>[8x]MAELACFCYPHLENDSYKFIPFNNLAIKAMLTAKVDKKDMDKFYDSIIYGIAPPPQFKKRYNTNDNSRGMNFETIMFTKVAMLICEALNSLKVTQANVSNVLSRVVSIRHLENLVIRKENPQDILFHSKDLLLKSTLIAIGQSKEIETTITAEGGEIVFQNAAFTMWKLTYLEHQLMPILDQNFIEYKVTLNEDKPISDVHVKELVAELRWQYNKFAVITHGKGHYRIVKYSSVANHADRVYATFKSNVKTGVNNDFNLLDQRIIWQNWYAFTSSMKQGNTLDVCKRLLFQKMKPEKNPFKGLSTDRKMDEVS

In RVs, the viral RNA chaperone protein NSP2 facilitates sequence-specific, intersegment RNA–RNA interactions to ensure robust assembly of complete viral genomes. NSP2 is a multivalent, nonspecific RNA chaperone with high nanomolar affinity for single-stranded (ss) RNA. The CTR of NSP2 consists of a flexible linker (residues 295 through 304) that tethers an α-helix (C-terminal helix, CTH) to NSP2core (i.e., residues 1 through 294). The CTH is ampholytic, containing highly conserved, positively (Arg307, Lys308) and negatively charged (Asp306, Asp310, and Glu311) residues.

To visualize the CTR conformation in solution, we determined a cryo-EM three-dimensional (3D) reconstruction of full-length NSP2 (henceforth referred to as NSP2) at a global resolution of 3.9 Å. Due to intrinsic flexibility, the linker region was poorly resolved. We analyzed our atomic model of NSP2 to evaluate the distances between acidic residues within the CTR and the basic, RNA-binding residues localized to flexible loops within the RNA-binding grooves. The distances (∼10 to 30 Å) between acidic residues within the CTR and the RNA-interacting residues are incongruent with a direct competition model.Sucrose import from photosynthetic tissues into the phloem is mediated by transporters from the low-affinity sucrose transporter family (SUC/SUT family). Whereas the SWEET facilitators efflux sugars, active loading depends on SUCs that use the plasma membrane proton motive force to drive uptake of sucrose for accumulation, with concentrations reaching as high as 1.3 molar in the phloem. SUCs are part of the Glycoside-Pentoside-Hexuronide (GPH):cation symporter family that belongs to the Major Facilitator Superfamily (MFS). SUC1 is predominantly expressed in reproductive organs, trichomes and roots, where it localizes in the plasma membrane and is required for proper pollen function.

Here we present the structure of the sucrose–proton symporter, Arabidopsis thaliana SUC1, in an outward open conformation at 2.7 Å resolution, together with molecular dynamics simulations and biochemical characterization. In the asymmetrical unit, SUC1 forms a non-physiological inverted dimer, with both monomers in the same conformation (root mean square deviation (r.m.s.d.) of Cɑ atoms = 0.1 Å). Overall, SUC1 adopts the canonical MFS transporter fold with twelve transmembrane helices arranged into two pseudosymmetrical halves consisting of two six-helix domains, the N-terminal domain (N domain, M1–M6) and C-terminal domain (C domain, M7–M12). Extracellularly, a short helical region (named extracellular helical region (EHR)), which also has clear amphipathic properties, is present in the loop connection between M5 and M6. The EHR is anchored to the side of the N domain by a disulfide bridge between the strictly conserved residues Cys216 and Cys220. The structure captures SUC1 in an outward open conformation with a conserved electrostatic network between the N and C domains at the cytosolic side. A large and clearly defined V-shaped cavity, which spans approximately two thirds of the membrane plane between the N and C domain, is open to the extracellular side. Overall, the cavity is electronegative, but it becomes electropositive towards the enclosing bottom. Despite the presence of sucrose during crystallization, no defined density for sucrose binding can be observed in the cavity. In the transmembrane domains of SUC1, the only acidic residue is Asp152(M4), which is strictly conserved in SUCs and therefore the prime candidate as the proton donor/acceptor residue during symport. Asp152 is exposed to the cavity solvent without any close contacts to other residues.

>MGGAYETEKPTKDAAALETQSPEDFDQPSPLRKIISVASIAAGVQFGWALQLSLLTPYVQLLGIPHKWSSLIWLCGPVSGMIVQPIVGFHSDRCRSKFGRRRPFIATGAALVAVAVFLIGYAADFGYKMGDKLEEKVKVRAIGIFALGFWILDVANNTLQGPCRAFLADLAAGDAKRTRVANAFFSFFMAVGNVLGYAAGSYTNLHKMFPFTMTKACDIYCANLKTCFFLSITLLLIVTVTSLWYVNDKQWSPPPRNADDDEKTSSVPLFGEIFGAFKVMKRPMWMLLIVTALNWIAWFPFLLFDTDWMGREVFGGDSDGNERSKKLYSLGVQSGAMGLMFNSIVLGFMSLGVEWIGRKLGGAKRLWGIVNFILAAGLAMTVLVTKFAEDHRKTAGDLAGPSASVKAGALSLFAVLGIPLAITFSTPFALASIFSSCSGAGQGLSLGVLNLAIVIPQMIVSLGGGPFDALFGGGNLPAFIVAAIAAAISGVLALTVLPSPPPDAPKATTMGGFHGLVPR[2x]>MLKLGVIGTGAISHHFIEAAHTSGEYQLVAIYSRKLETAATFASRYQNIQLFDQLEVFFKSSFDLVYIASPNSLHFAQAKAALSAGKHVILEKPAVSQPQEWFDLIQTAEKNNCFIFEAARNYHEKAFTTIKNFLADKQVLGADFN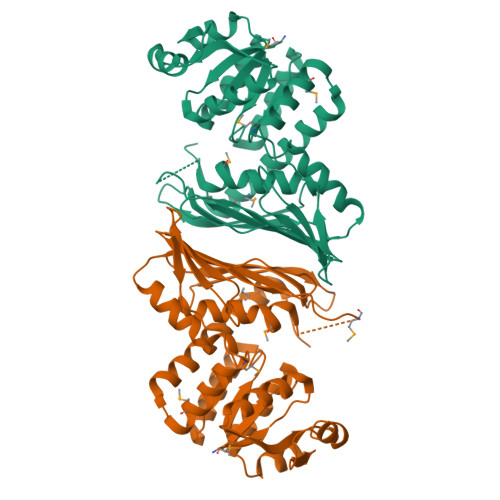YAKYSSKMPDLLAGQTPNVFSDRFAGGALMDLGIYPLYAAVRLFGKANDATYHAQQLDNSIDLNGDGILFYPDYQVHIKAGKNITSNLPCEIYTTDGTLTLNTIEHIRSAIFTDHQGNQVQLPIQQAPHTMTEEVAAFAHMIQQPDLNLYQTWLYDAGSVHELLYTMRQTAGIRFEAEK[2x]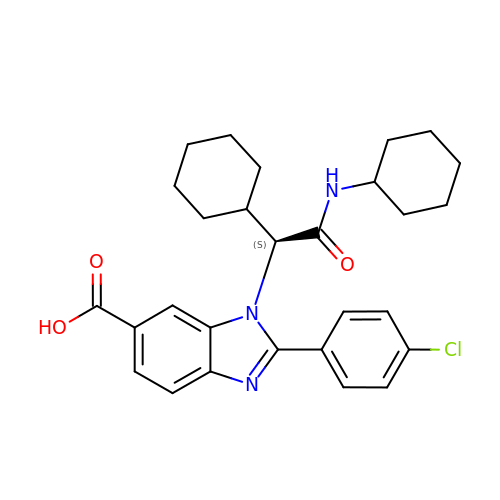2-(4-chlorophenyl)-1-[(1S)-1-cyclohexyl-2-(cyclohexylamino)-2-oxoethyl]-1H-benzimidazole-6-carboxylic acid | C28 H32 Cl N3 O3 | BGTNSFBYQMPTOK-VWLOTQADSA-N In the family of triosephosphate isomerases (TIM) there is a strictly conserved cysteine, which is located near the end of the β-strand 5, forming part of the hydrophobic core of the (β/α)8 barrel-structure displayed by these enzymes. The sulfur atom of this invariant cysteine (Cys126, according to the sequence numbering of Saccharomyces cerevisiae TIM, ScTIM) is located at van der Waals distance from one of the oxygen atoms of the catalytic Glu165; yet, substitution of Cys126 by Ala or Ser only slightly affects the activity of ScTIM. Mutation of Cys126 has, on the other hand, sound effects on the stability of the native yeast TIM dimer. The structure of C126S ScTIM shows the canonical features conserved for this protein, with the common (β/α)8 TIM-barrel fold consisting of a barrel of eight β-strands surrounded by helices.

To find out what structural modifications occur in the molecule of yeast TIM when Ser replaces Cys126, we determined the crystal structure of the C126S mutant at 1.86 Å resolution. The structure showed the presence of the substrate analog 2-phosphoglycolate (PGA) in monomer A only. The electron density observed at the active site of monomer B did not account for an intact PGA; therefore, we interpreted this density as a sulfate ion and glycerol with occupancies of 1.0. It is important to mention that the catalytic loop or loop 6 presents a “closed” conformation in monomer A (with PGA), and the “open” conformation in monomer B, which contains glycerol and a sulfate ion, a situation that has been observed before for P. falciparum TIM in the presence of 2-phosphoglycerate (2PG). In our structure, PGA is bound to the catalytic site in monomer A with a tight hydrogen-bond network including NZ-Lys12, NE2-His95, OE2-Glu165, N-Gly171, N-Ser211, N-Gly232 and N-Gly233, which are structurally conserved among different structures. The main local changes around the mutation include the presence of several water molecules, not observed in the wild type enzyme (respectively). In monomer A two water molecules establish three hydrogen bonds with Ser126, whereas in monomer B three water molecules form four hydrogen bonds with this residue. In contrast, Cys126 in the wild-type protein interacts with a single water molecule. The key point seems to be that, due to its highly polar nature, the OH group of the Ser residue turns out from the interior of the β-barrel and, in its new environment, establishes hydrogen bonds with Glu165 and two water molecules. This new rotamer orientation apparently gives rise to penetration of additional water molecules that likely modify the polar/apolar nature of an interior region of the molecule. Furthermore, a long stretch of residues (Glu132-Val142), which becomes unstable, as indicated by MD simulations, may be the origin of the faster unfolding of the C126S mutant with respect to the wild-type Sc-TIM.

>[2x]MARTFFVGGNFKLNGSKQSIKEIVERLNTASIPENVEVVICPPATYLDYSVSLVKKPQVTVGAQNAYLKASGAFTGENSVDQIKDVGAKWVILGHSERRSYFHEDDKFIADKTKFALGQGVGVILSIGETLEEKKAGKTLDVVERQLNAVLEEVKDWTNVVVAYEPVWAIGTGLAATPEDAQDIHASIRKFLASKLGDKAASELRILYGGSANGSNAVTFKDKADVDGFLVGGASLKPEFVDIINSRN> HMGLRGDYFDNIDLTNFKLTRVDKTIDFFWGVNSPAKEIRNDESYSVRWTGKIRPLYSEEYTFYISRDNGVRLWIDNKLIIDKWDNLVGLDEMGKIYLEAGKLYDIKLEYFNNTGNGFVKLEWSSASTVRSIVPTECLYPAEPKHYGSSIPGKGIGLFYEYFDEDNLTNPKEKGIDSVIDFNWGVGSPSKSINQDQKFSVRWTGFIQVPYDGDYVFYVSYDDGASLWIDRQLLID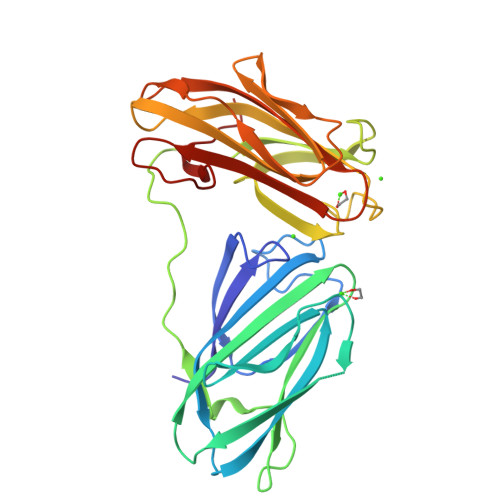KWTASEINTAKTEAISLKAGQRVEVMLLYRNTGLAGSIRLEWEGPGIERSVVPQSCLYPR>[2x]MSLAIQNPYTAYQQNSVNTATPGELTLMLYNGCLKFIRLAAQAIENDDMERK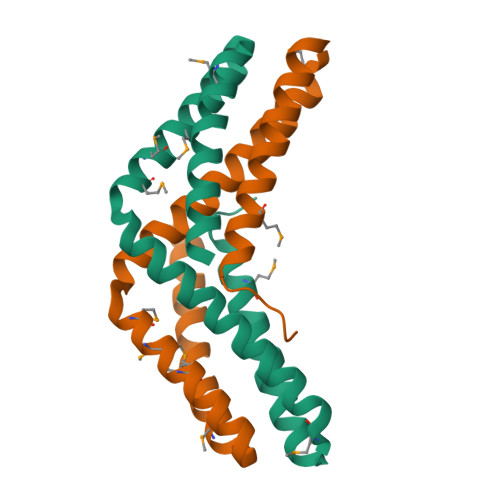NENLIKAQNIIQELNFTLNRNIELSASMGAMYDYMYRRLVQANIKNDTGMLAEVEGYVTDFRDAWKQAIQSERKDRHGSGGIAEGGSHHHHHH> MESKKRQWALEDFEIGRPLGKGKFGNVYLAREKQSKFILALKVLFKAQLEKAGVEHQLR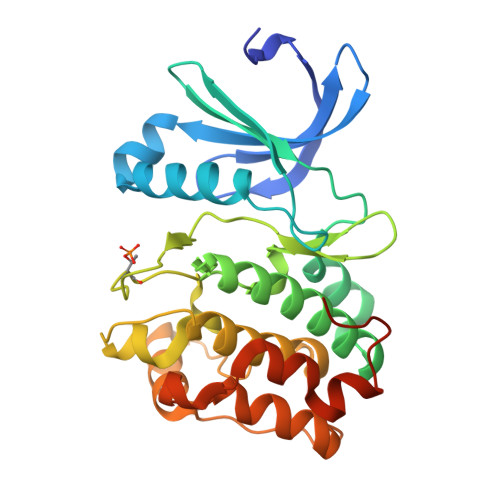REVEIQSHLRHPNILRLYGYFHDATRVYLILEYAPLGTVYRELQKLSKFDEQRTATYITELANALSYCHSKRVIHRDIKPENLLLGSAGELKIADFGWSVHAPSSRRTTLAGTLDYLPPEMIEGRMHDEKVDLWSLGVLCYEFLVGKPPFEANTYQETYKRISRVEFTFPDFVTEGARDLISRLLKHNPSQRPMLREVLEHPWITANSSKPSNAQNKESASKQS>[2x]MAKHATPLLDQLQSGPWPSFVADIKEEAERRHSNQDNVEYQIPVDVCDDLLGILELKYSDGTTHWKHGGIVGVFGYGGGVIGRYCDQPQMFPGVAHFHTVRVAQPAGMYYTTDFLKQLCDLWDMRGSGLTNMHGATGDIVLLGTTTPQLEEFYFELTHKMNNDLGGSGSNLRTPASCLGDSRCEWACYDAQELCYQMTQEYQDELHRPAFPYKFKFKFDGCPNGCVASIARSDMSFIGTWRDDIRIDQEAVAAYVGGEIQPNGGAHSGKDWGAFDIQKEVIDLCPTECMWMEDGKLQINNRECTRCMHCLNVMPRALRIGNDRGLSILVGAKAPILDGAQMGSLLVPFIKVEDPYDEIKEIIEGIWEWWMEEGKNRERLGELIKRQGLAKAIAAVGLTPVPQHVMEPR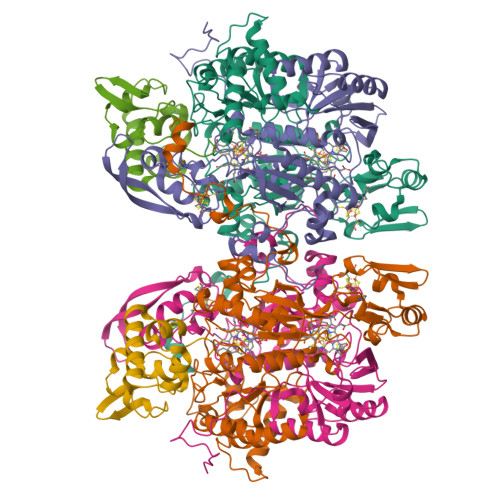HNPYIFWKEKDVEGGWDRDIADYRKHHQR;>[2x]MAFVSSGYNPEKPMENRISDIGPRHASDFFPPVIAKNKGQWLWHEICEPGILMHKAESGDEVYTVRCGGARLMSVGHIREICAIADKFCGGHLRFTTRNNIEFMVTTLDEAKKLKEYLNAQKFEGGSFKFPVGGTGAGITNIVHTQGWVHCHTPATDASGTVKVVLDELFEEFGQMRMPAQVRISMACCLNMCGAVHCSDIAILGYHRKPPVIDHEWLDNLCEIPLAVAACPVGAIRPTKKEIVTEKGETKTVNTVAIKNERCMFCGNCYTMCPSLPLSDQTGDGLVIMAGGKVSNRISNPKFSKVVVAFIPNEPPRWPRLASVIRQIVEAYAADARKYERVGDWAERIGWERFFEKCELDFSIHMIDDFRDPAYYTWRQTTNFKF;>MAMIEFKGKSFEIDEDGFLLKFEDWGPEWAEYVKESEGISEITEAHQQILDFLQDYYKKNGIAPMVRILSKSTGYKLKQIYELFPSGPGKGACKMAGLPKPTGCV[2x]>MKTRINYAKASPEAFKAVMALENYVQSSGLEHRFIHLIKLRASIINGCAFCVDMHVKESRHDGLSEQWINLMSVWRESPVYTEQERALL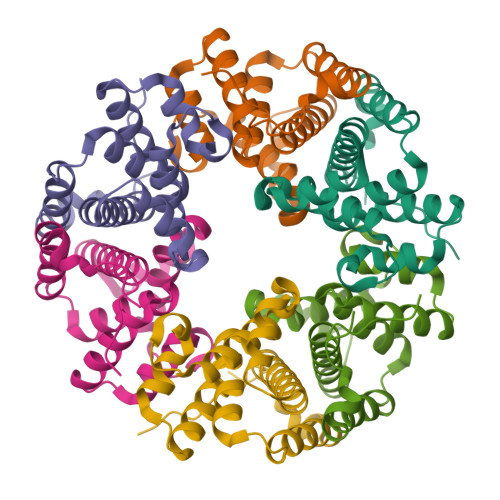GWVDAVTKIAETGAPDDAFETLRAHFSDEEIVKITVAIGAINTWNRIAVGFRSQHPVEAAAKAA[6x]> S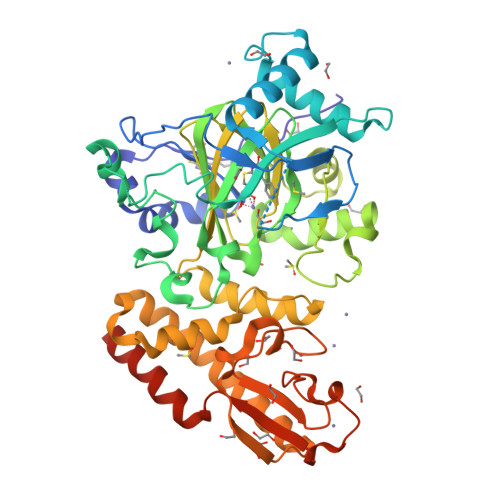MFLPPPECPVFEPSWEEFADPFAFIHKIRPIAEQTGICKVRPPPDWQPPFACDVDKLHFTPRIQRLNELEAQTRVKLGGGGARDYTLRTFGEMADAFKSDYFNMPVHMVPTELVEKEFWRLVSTIEEDVTVEYGADIASKEFGSGFPVRDGKIKLSPEEEEYLDSGWNLNNMPVMEQSVLAHITADICGMKLPWLYVGMCFSSFCWHIEDHWSYSINYLHWGEPKTWYGVPGYAAEQLENVMKKLAPELFVSQPDLLHQLVTIMNPNTLMTHEVPVYRTNQCAGEFVITFPRAYHSGFNQGFNFAEAVNFCTVDWLPLGRQCVEHYRLLHRYCVFSHDEMICKMASKADVLDVVVASTVQKDMAIMIEDEKALRETVRKLGVIDSERMDFELLPDDERQCVKCKTTCFMSAISCSCKPGLLVCLHHVKELCSCPPYKYKLRYRYTLDDLYPMMNALKLRAESYNEWALNVNEALEAKI>AGLENTDHTNNEHRLTQLLSIAEECETLDRLKQLVDSGRIFTAYNGFEPSGRIHIAQALITVMNTNNMIECGGQMIIYIADWFAKMNLKMNGDINKIRELGRYFIEVFKACGINLDGTRFIWASEFIASNPSYIERMLDIAEFSTISRVKRCCQIMGRNESDCLKASQIFYPCMQAADVFELVPEGIDICQLGIDQRKVNMLAIEYANDRGLKIPISLSHHMLMSLSGPKKKMSKSDPQGAIFMDDTEQEVSEKISRAYCTDETFDNPIFEYIKYLLLRWFGTLNLCGKIYTDIESIQEDFSSMNKRELKTDVANYINTII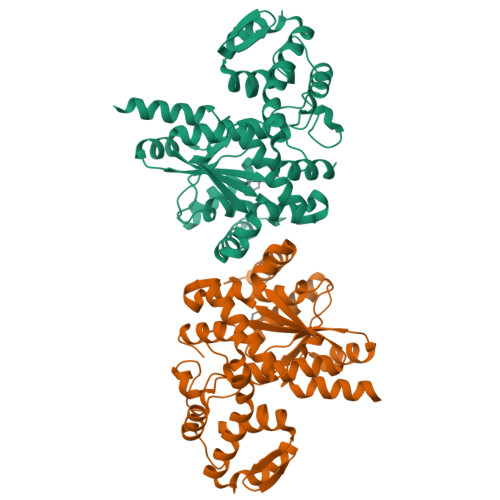DLVREHFKKPELSELLSNVKSYQQPSK[2x]The Eph receptors are the largest receptor tyrosine kinase family, and together with their cell surface-anchored ephrin ligands represent an important cell-cell communication system that regulates a multitude of physiological and pathological processes. The intracellular portion of the Eph receptors includes a juxtamembrane segment, the tyrosine kinase domain, a linker, a sterile alpha motif (SAM) domain, and a short C-terminal tail containing a PDZ domain-binding motif. EphA2 promotes cancer malignancy through a poorly understood non-canonical form of signaling involving serine/threonine phosphorylation of the linker connecting its kinase and SAM domains. The kinase-SAM linker contains a cluster of five serine/threonine residues that besides S897 include S892, T898, S899 and S901.

To determine whether the negative charges introduced by phosphorylation of the linker might affect the kinase-SAM domain arrangement, we solved the structures of two EphA2 phosphomimetic mutants. In the second EphA2 mutant, we replaced only S901 with glutamic acid. The EphA2 S901E structure is essentially identical to the WT structure, in agreement with the lack of definition of residue S901 in the structures and suggesting that S901 phosphorylation alone does not significantly affect the conformation of the EphA2 intracellular region.

>[2x]GPGDPHTYEDPNQAVLKFTTEIHPSCVTRQKVIGAGEFGEVYKGMLKTSSGKKEVPVAIKTLKAGYTEKQRVDFLGEAGIMGQFSHHNIIRLEGVISKYKPMMIITEYMENGALDKFLREKDGEFSVLQLVGMLRGIAAGMKYLANMNYVHRDLAARNILVNSNLVCKVSDFGLSRVLEDDPEATYTTSGGKIPIRWTAPEAISYRKFTSASDVWSFGIVMWEVMTYGERPYWELSNHEVMKAINDGFRLPTPMDCPSAIYQLMMQCWQQERARRPKFADIVSILDKLIRAPDSLKTLADFDPRVSIRLPSTSGEEGVPFRTVSEWLESIKMQQYTEHFMAAGYTAIEKVVQMTNDDIKRIGVRLPGHQKRIAYSLLGLKDQVNTVGIPI> XIWLAQGGRRLGDEINAYYAR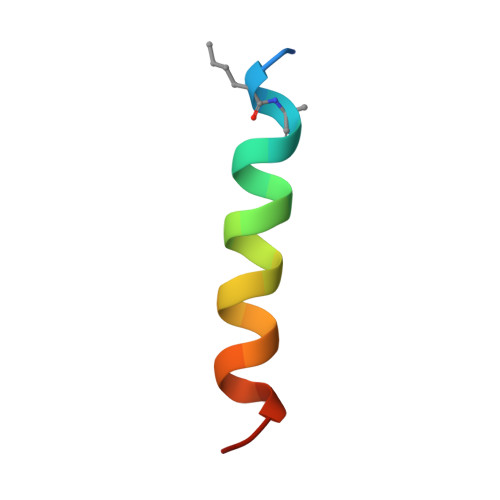RX>[4x]MGIPADNLQSRAKASFDTRVAAAELALNRGVVPSFANGEELLYRNPDPDNTDPSFIASFTKGLPHDDNGAIIDPDDFLAFVRAINSGDEKEIADLTLGPARDPETGLPIWRSDLANSLELEVRGWENSSAGLTFDLEGPDAQSIAMPPAPVLTSPELVAEIAELYLMALGREIEFSEFDSPKNAEYIQFAIDQLNGLEWFNTPAKLGDPPAEIRRRRGEVTVGNLFRGILPGSEVGPYLSQYIIVGSKQIGSATVGNKTLVSPNAADEFDGEIAYGSITI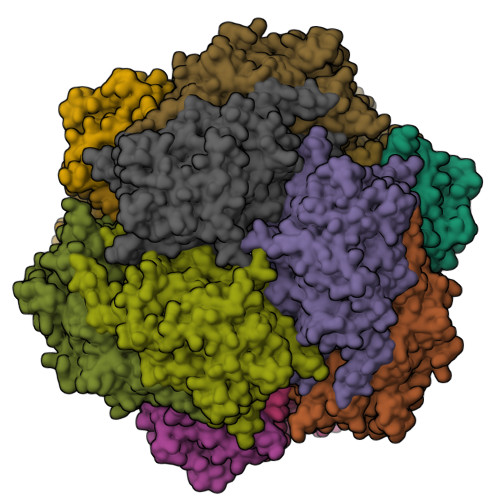SQRVRIATPGRDFMTDLKVFLDVQDAADFRGFESYEPGARLIRTIRDLATWVHFDALYEAYLNACLILLANGVPFDPNLPFQQEDKLDNQDVFVNFGSAHVLSLVTEVATRALKAVRYQKFNIHRRLRPEATGGLISVNKIAAQKGESIFPEVDLAVEELGDILEKAEISNRKQNIADGDPDPDPSFLLPMAFAEGSPFHPSYGSGHAVVAGACVTILKAFFDSGIEIDQVFEVDKDEDKLVKSSFKGTLTVAGELNKLADNIAIGRNMAGVHYFSDQFESLLLGEQVAIGILEEQSLTYGENFFFNLPKFDGTTIQI>RLIHVSRCEMGTSTHRCWPRPCDTSSDEPISFWPPFENTPNVIVSFGMLDVDNSNNLRVNSSADDVTVGGFT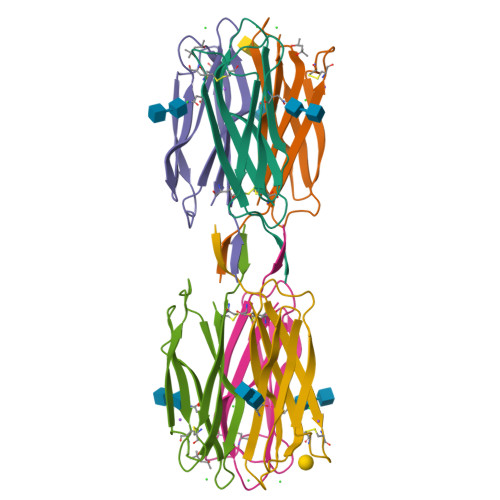LHYNSWYTTTVWNYKLIWIACD[6x]>[2x]MEQQLTIEMIADAFSYDITGFDCGEEALNTFLKEHLKRQHDGQILRGYALVSGDTVPRLLGYYTLSGSCFERGMLPSKTQQKKIPYQNAPSVTLGRLAIDKSVQGQGWGE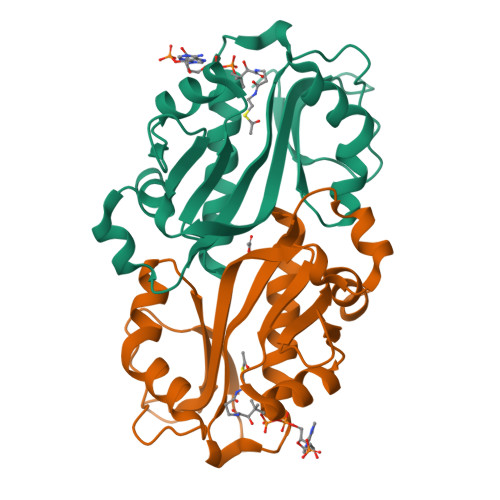MLVAHVMRVVWGASKAVGIYGLFVEALNEKAKAFFLRLGFIQLVDENSNLLFYPTKSIEQLFTDDES> MTTQQLKEKISKIIDNFSGIRVVFTTTANELKLSRIEGSALNSIAEGFIDKIKEDIINNEDLTSPLLSNFDDRKNALFKFDYEQYPEEFNKITQAIAIPPNSQDYYNPLNKFTDVKGIIILISGDNKCLALYKNKTNLAVLRNSRKMFNLVPDPDGYLKQLPNEILRLDFNYDLFSIGEDFYIKNHKTLETQMKFHQVIEAQAVIALNSLRDSLLIEDISGLEKSSREISFA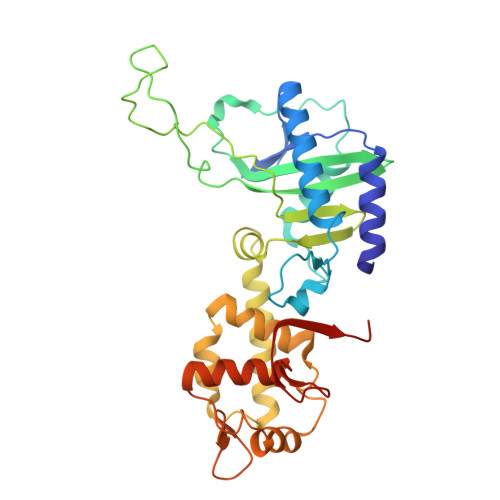RKLAKISKHSPVLGKIDTKTIIDYVSQHKYLSAILQINEAGDKLLIKTKTSQKHFIKLMSDDYLQSDLTKIIYMSIAKDRLDEHHHHHH> KPVTVKLVDSQATMETRSLFAFMQEQRRHSIMFGHQHETTQGLTITRTDGTQSDTFNAVGDFAAVYGWDTLSIVAPKAEGDIVAQVKKAYARGGIITVSSHFDNPKTDTQKGVWPVGTSWDQTPAVVDSLPGGAYNPVLNGYLDQVAEWANNLKDEQGRLIPVIFRLYHANTGSWFWWGDKQSTPEQYKQLFRYSVEYLRD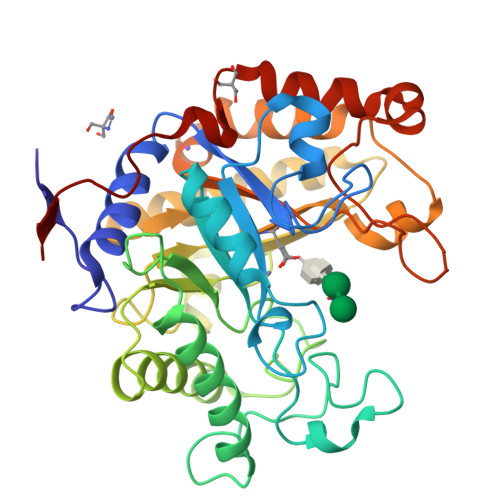VKGVRNFLYAYSPNNFWDVTEANYLERYPGDEWVDVLGFDTYGPVADNADWFRNVVANAALVARMAEARGKIPVISEIGIRAPDIEAGLYDNQWYRKLISGLKADPDAREIAFLLVWRNAPQGVPGTQVPHYWVPANRPENINNGTLEDFQAFYADEFTAFNRDIEQVYQRPTLI>MNSYPIVLVHGFMGWGRNEVLGLKYWGGITDYEQELSSYGYTAYTATVGPVSSNWDRACELYAYIKGGTVDYGHAHSTQKGHSRYGRTYPGLYPEWGNLTTEGKVNKIHLVAHSMGGQTVRTLVQLLKEGSEEERNTTPSQLSSLFAGGKSWVHSITTIASPHDGTTLADGINIFGDFAKNLVASLASFTGAGEKLIYDFKLDQWGLNRKSGESLTDYTNRVFNSAIWNSTNDLANWDLSTDGARVLNQWVKAQSDIYYFSYSTCATVPSILTSNELPHVIYMTPLLYPFGRFIGSYTRNEQGRVIIDNSWKPNDGVVNTISQNGPKIWSSDKIVNYNGVPQIGKWNSMPLLDTIDHMDAC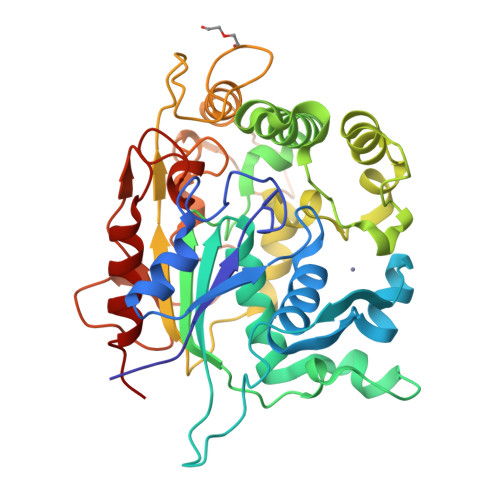GIGTNALTLSWYKGLAEKLSQLTISN[2x]An alternative, promising approach involves protein capsids, such as encapsulins, which can be viewed as genetically encoded enzyme encapsulation, and is particularly suitable for immobilization or within physiological conditions. The capsids, comprised of 60–240 subunits arranged in an icosahedral structure, engage with a conserved C-terminal encapsulin localization sequence (ELS), or a more extended N-terminal encapsulation-mediating domain, found on the guest protein. Our study showcases the encapsulation of the nitroreductase NfsB, which we produced as a fused dimer, within encapsulins.

To investigate the assembly of the Enc{tdNfsB} construct in detail, we performed single-particle cryo-EM analysis of the purified capsids. The overall resolution of the encapsulin icosahedral shell was determined to be 2.22 Å based on the gold standard Fourier Shell Correlation (FSC) 0.143 threshold (ESI†). The calculated diameter of the shell was 24.0 nm, which correlates well with the expected solution hydrodynamic diameter and has a calculated internal volume of 3000 nm3. The crystal and cryo-EM structures of encapsulins from close homologs, have multiple openings in their capsid shells, including a threefold pore and an five-fold pore. The cryo-EM map in this area was ambiguous however and appears to be the superimposition of flexible states. To resolve this, the pentameric subunit was examined by 3-D classification and resulting volumes were refined using local refinement without symmetry constraints. This isolation a series of volumes that could be categorized as open, closed or uninterpretable. The open and closed particles were pooled and refined to yield complete, unambiguous maps (ESI†). The primary drive of this is a shift in the pore forming loop (measuring 3.84 Å between the displaced His188 alpha carbon, see attached movies M1 and M2). The underlying cause of this movement is unclear and may represent an equilibrium of states when resting at cellular pH or could be a result of different packing states within the particles stacks.

>[60x]MNNLYRDLAPITESAWAEIELEATRTFKRHIAGRRVVDVSGPNGPTTASVSTGHLLDVSPPGDGVIAHLRDAKPLVRLRVPFTVARRDIDDVERGSQDSDWDPVKDAAKKLAFVEDRAIFEGYAAASIEGIRSSSSNPALALPDDAREIPDVIAQALSELRLAGVDGPYSVLLSAETYTKVSETTAHGYPIREHINRLVDGEIIWAPAIDGAFVLSTRGGDFDLQLGTDVSIGYLSHDAEVVHLYMEETMTFLCYTAEASVALTPELWSHPQFEK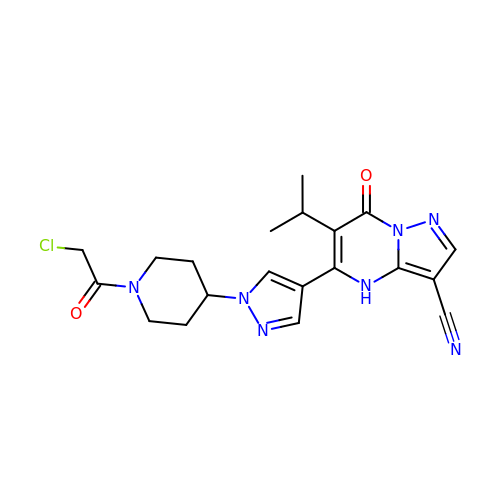5-[1-[1-(2-chloranylethanoyl)piperidin-4-yl]pyrazol-4-yl]-7-oxidanylidene-6-propan-2-yl-4~{H}-pyrazolo[1,5-a]pyrimidine-3-carbonitrile | C20 H22 Cl N7 O2 | UFTLGLOWZBFFND-UHFFFAOYSA-N> QDVRVQVLPEVRGQLGGTVELPCHLLPPVPGLYISLVTWQRPDAPANHQNVAAFHPKMGPSFPSPKPGSERLSFVSAKQSTGQDTEAELQDATLALHGLT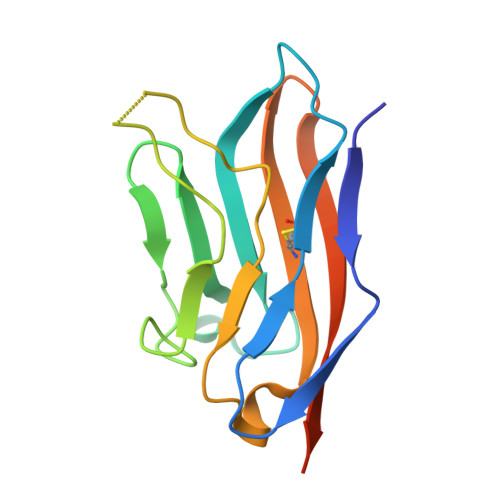VEDEGNYTCEFATFPKGSVRGMTWLRVLVPRGSGHHHHHH> VMTMRGLLVGAMQPFHRGHLQVIKSILEEVDELIICIGSAQLSHSIRDPFTAGERVMMLTKALSENGIPASRYYIIPVQDIECNALWVGHIKMLTPPFDRVYSGNPLVQRLFSEDGYEVTAPPLFYRDRYSGTEVRRRMLDDGD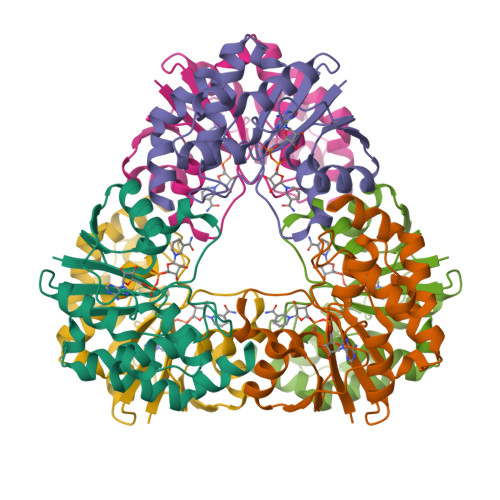WRSLLPESVVEVIDEINGVERIKHLAKKEVSELGGIS>[2x]MKHLEEKTLSTRQIFKGRYLKIEQDQVQAPDGRTYTREYILHPGAAMMIPLLPNGNVVMIHQYRHAVKKVFLEFPAGKRDHNEETLLTAKRELLEETGYEAKDWKFLTTIHPVIGYSNEHIDLYLARDLTHLEQRLDQGQFIEVVEVKPADLMQLVLEGKVSDVKTQIGAFWLDKFLRGEWN

Of particular interest is the Bdellovibrio bacteriovorus HD100 nucleoside diphosphate sugar (NDPS) hydrolase Bd3179 because it appears to have some of the characteristics of the Escherichia coli adenosine diphosphate ribose (ADPR) hydrolase and the guanosine diphosphate mannose (GDPM) hydrolase. Bd-NDPSase is a homodimer whose monomers are related by a non-crystallographic 2-fold axis. Each monomer comprises an N-terminal and a Nudix domain. Phosphate release assays revealed that among the nucleoside diphosphate sugars hydrolyzed by Bd-NDPSase, its highest relative activity was with GDPM.

Bd-NDPSase crystals soaked with UDPG displayed electron density that could be interpreted as a glucose molecule in each active site of the asymmetric unit. Modeling of glucose, sulfate, and glycerol molecules in the unbiased electron density revealed that these molecules are located within hydrogen bonding distance of catalytic residues. R64 makes a hydrogen bond with the sulfate and glucose molecules through its guanidinium side chain. Water molecules mediate the interactions of these molecules with other key residues such as E96, Q140, and K165. The glucose molecule is shifted toward the expected position of the phosphate of a phosphohexose product. The proposition that E140 functions in catalysis is strengthened by the fact that substitution by glutamine renders the enzyme catalytically inactive, as evidenced by both relative activity assays and kinetic assays.>MNPAAEAEFNILLATDSYKVTHYKQYPPNTSKVYSYFECREKKTENSKLRKVKYEETVFYGLQYILNKYLKGKVVTKEKIQEAKDVYKEHFQDDVFNEKGWNYILEKYDGHLPIEIKAVPEGFVIPRGNVLFTVENTDPECYWLTNWIETILVQSWYPITVATNSREQKKILAKYLLETSGNLDGLEYKLRDFGYRGVSSQETAGIGASAHLVNFKGTDTVAGLALIKKYYGTKDPVPGYSVPAAEHSTITAWGKDHEKDAFEHIVTQFSSVPVSVVSDSYDIYNACEKIWGEDLRHLIVSRSTQAPLIIRPDSGNPLDTVLKVLEILGKKFPVTENSKGYKLLPPYLRVIQGDGVDINTLQEIVEGMKQKMWSIENIAFGSGGGLLQKLTRDLLNCSFKCSYVVTNGLGINVFKDPVADPNKRSKKGR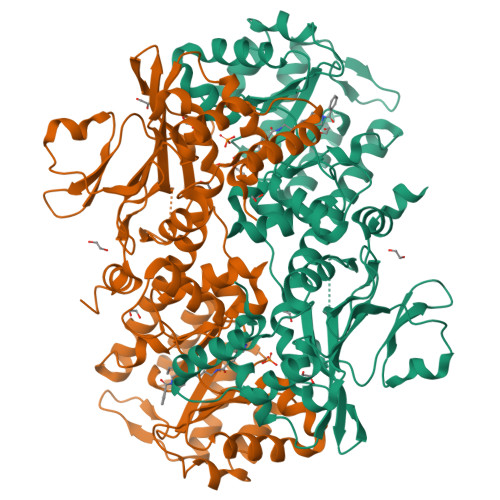LSLHRTPAGNFVTLEEGKGDLEEYGQDLLHTVFKNGKVTKSYSFDEIRKNAQLNIELEAAHHLEHHHHHHHH[2x]>ARLGARPCGLRELEVRVSELGLGYASDETVLFRYCAGACEAAARVYDLGLRRLRQRRRLRRERVRAQPCCRPTAYEDEVSFLDAHSRYHTVHELSARECACV[4x];>[4x]SSLQGPELHGWRPPVDCVRANELCAAESNCSSRYRTLRQCLAGRDRNTMLANKECQAALEVLQESPLYDCRCKRGMKKELQCLQIYWSIHLGLTEGEEFYEASPYEPVTSRLSDIFRLASIFSGTGADPVVSAKSNHCLDAAKACNLNDNCKKLRSSYISICNREISPTERCNRRKCHKALRQFFDRVPSEYTYRMLFCSCQDQACAERRRQTILPSCSYEDKEKPNCLDLRGVCRTDHLCRSRLADFHANCRASYQTVTSCPADNYQACLGSYAGMIGFDMTPNYVDSSPTGIVVS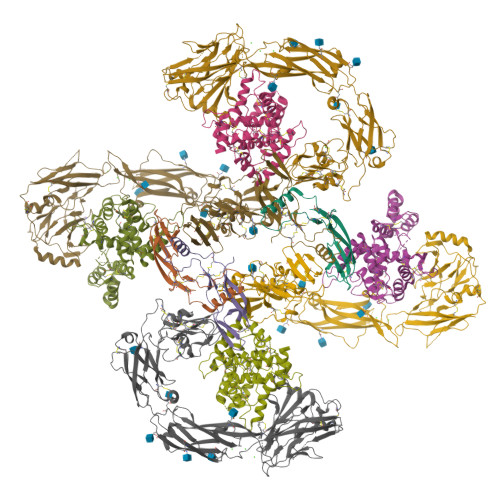PWCSCRGSGNMEEECEKFLRDFTENPCLRNAIQAFGNGTDVNGTHHHHHHHH;>[4x]LYFSRDAYWEKLYVDQAAGTPLLYVHALRDAPEEVPSFRLGQHLYGTYRTRLHENNWICIQEDTGLLYLNRSLDHSSWEKLSVRNHGFPLLTVYLKVFLSPTSLREGECQWPGCARVYFSFFNTSFPACSSLKPRELCFPETRPSFRIRENRPPGTFHQFRLLPVQFLCPNISVAYRLLEGEGLPFRCAPDSLEVSTRWALDREQREKYELVAVCTVHAGAREEVVMVPFPVTVYDEDDSAPTFPAGVDTASAVVEFKRKEDTVVATLRVFDADVVPASGELVRRYTSTLLPGDTWAQQTFRVEHWPNETSVQANGSFVRATVHDYRLVLNRNLSISENRTMQLAVLVNDSDFQGPGAGVLLLHFNVSVLPVSLHLPSTYSLSVSRRARRFAQIGKVCVENCQAFSGINVQYKLHSSGANCSTLGVVTSAEDTSGILFVNDTKALRRPKCAELHYMVVATDQQTSRQAQAQLLVTVEGSYVAEEAGCPLSCAVSKRRLECEECGGLGSPTGRCEWRQGDGKGITRNFSTCSPSTKTCPDGHCDVVETQDINICPQDCLRGSIVGGHEPGEPRGIKAGYGTCNCFPEEEKCFCEPEDIQDPLCDELCRGTHHHHHHHH>MRGSHHHHHHGSMPVAGSELPRRPLPPAAQERDAEPRPPHGELQYLGQIQHILRCGVRKDDRTGTGTLSVFGMRARYSLRDEFPLLTTKRVFWKGVLEELLWFIKGSTNAKELSSKGVKIWDANGSRDFLDSLGFSTREEGDLGPVYGFQWRHFGAEYRDMESDYSGQGVDQLQRVIDTIKTNPDDRRIIMCAWNPRDLPLMALPPCHALCQFYVVNSELSCQLYQRSGDMGLGVPFNIASYALLTYMIAHITGLKPGDFIHTLGDAHIYLNHIEPLKIQLQREPRPFPKLRILRKVEKIDDFKAEDF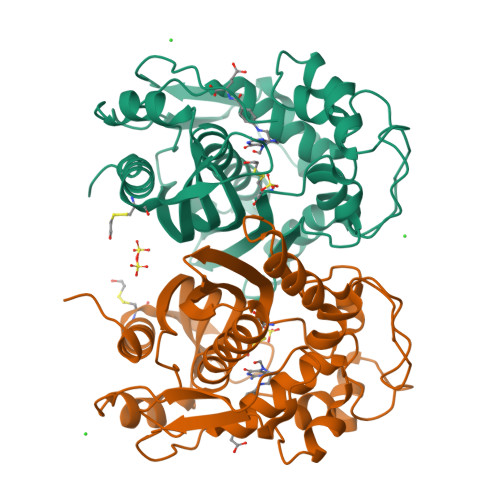QIEGYNPHPTIKMEMAV[8x]(1R,3R,7E,17beta)-17-{(2R,6S)-6-hydroxy-7-[(3S,5S,7S)-tricyclo[3.3.1.1~3,7~]dec-1-yl]hept-4-yn-2-yl}-2-methylidene-9,10-secoestra-5,7-diene-1,3-diol 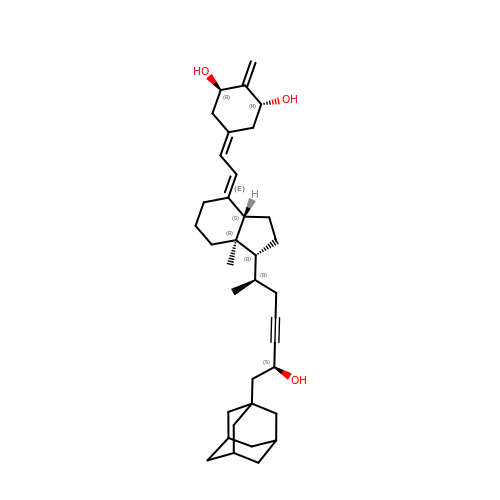| C36 H52 O3 | UFJLHOSCLNTAFF-OLECLGHFSA-N>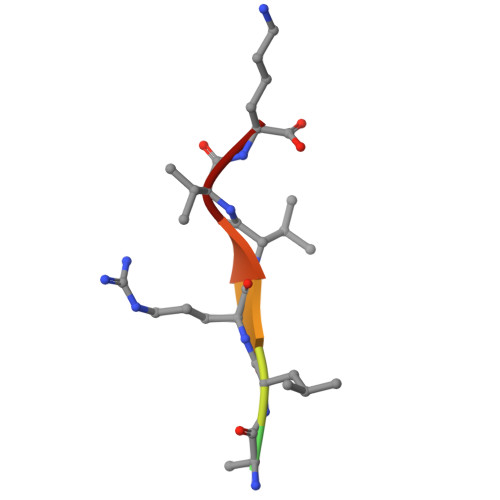 APALRVVK> RSWHYVEPKFLNKAFEVALKVQIIAGFDRGLVKWLRVHGRTLSTVQKKALYFVNRRYMQTHWANYMLWINKKIDALGRTPVVGDYTRLGAEIGRRIDMAYFYDFLKDKNMIPKYLPYMEEINRMRPADV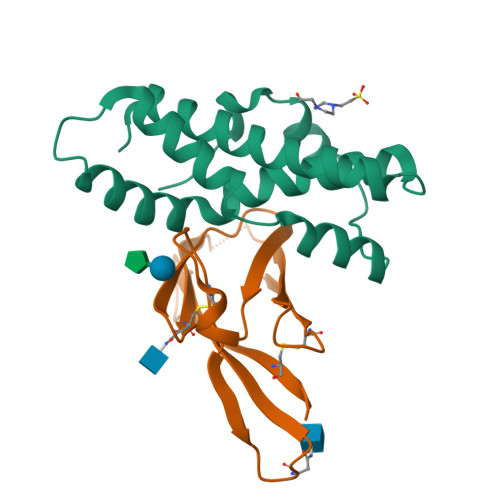PVKYMGK;> ETGAAADWDVYCSQDESIPAKFISRLVTSKDQALEKTEINCSNGLVPITQEFGINMMLIQYTRNELLDSPGMCVFWGPYSVPKNDTVVLYTVTARLKWSEGPPTNLSIQCYMPKSPVAPKLEHHHHHH>AKRLSIQQLAKAIANTLETPPQPKAGRRRNRRRQRSAVQQLPPIQAGISMAPSAQGAMVRIRNPAVSSSRGAITVLHCELTAEIGVTDSIVVSSELVMPYTVGTWLRGVADNWSKYSWLSVRYTYIPSCPSSTAGSIHMGFQYDMADTVPVSVNKLSNLRGYVSGQVWSGSAGLCFINNSRCSDTSTAISTTLDVSELGKKWYPYKTSADYATAVGVDVNIATDLVPARLVIALLDGSSSTAVAAGRIYDTYTIQMIEPTASALNL[3x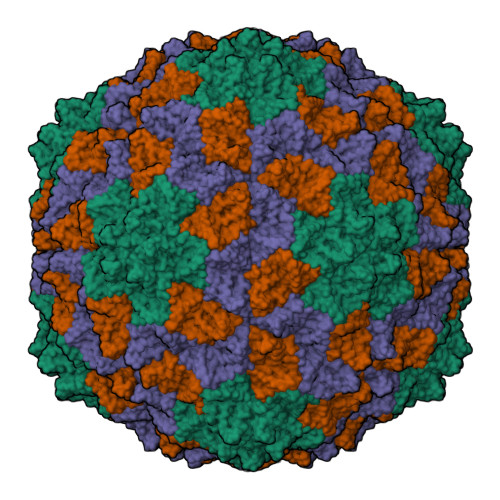]>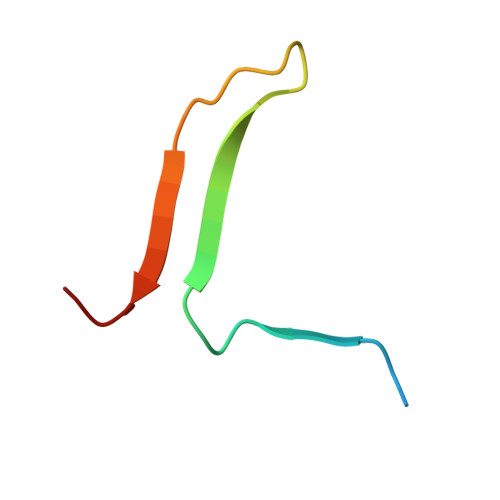 SALVETRTIVRFNRPFLMIIVPTDTQNIFFMSKVTNPKQA In order to understand the structural basis for the effect of N6‐methyladenine on k‐turn conformation, we have used X‐ray crystallography to investigate the structural effect of this modification on different base pairs involving adenine. Each species was formed by the hybridization of a self‐complementary strand that contains a 5‐bromocytosine nucleotide used to calculate phases for the diffraction in most cases. Crystallography reveals that N6‐methylation of adenine prevents the formation of trans Hoogsteen‐sugar A·G base pairs, explaining why the box C/D RNA cannot adopt its kinked conformation. More generally, our data indicate that sheared A·G base pairs (but not Watson–Crick base pairs) are more susceptible to disruption by N6mA methylation and are therefore possible regulatory sites.

We studied another duplex of sequence identical to that of the previous one, except that the G‐C base pairs flanking the central G·A pairs were replaced by G·U pairs. Two forms were synthesized, with and without N6‐methyladenine replacing the central adenine bases that oppose the guanine nucleotides. The unmodified RNA formed a fully basepaired helix, but in contrast to the previous sequence, the G·A pairs formed trans sugar‐Hoogsteen base pairs with two H‐bonds between GN2:AN7 (2.8 Å) and AN6:GN3 (3.4 Å). This is the same as the two trans sugar‐Hoogsteen G·A base pairs found in the core of the k‐turn. The flanking G·U pairs form trans base pairs connected by a single H‐bond GN2:UO4 (2.8 Å). Crystal structures of RNA duplexes in which guanine opposes adenine or N6‐methyladenine with flanking G·U base pairs.

>[2x]GCCGGAUGGC>[6x]GPGSMADPSLNNPVVIQATRLD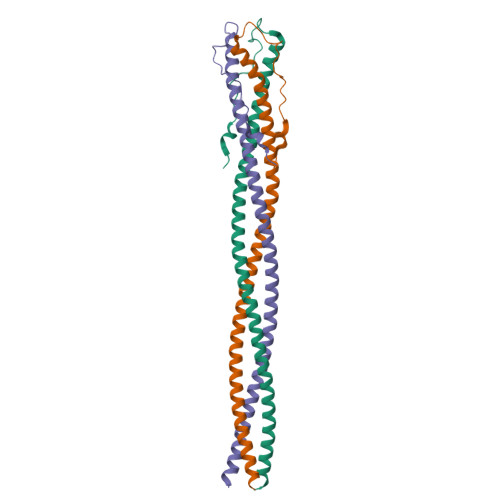ASILPRNVFSKSYLLYVIAQGTDVGAIAGKANEAGQGAYDAQVKNDEQDVELADHEARIKQLRIDVDDHESRITANTKAITALNVRVTTAEGEIASLQTNVSALDGRVTTAENNISALQADY GLUTATHIONYLSPERMIDINE 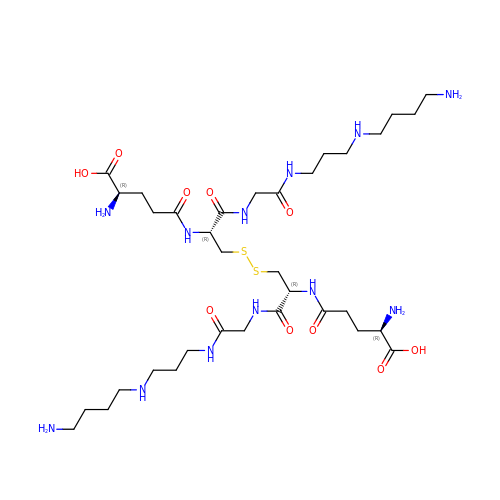DISULFIDE | C34 H66 N12 O10 S2 | HCMZDPYSWPSKSP-XPGKHFPBSA-N>[2x]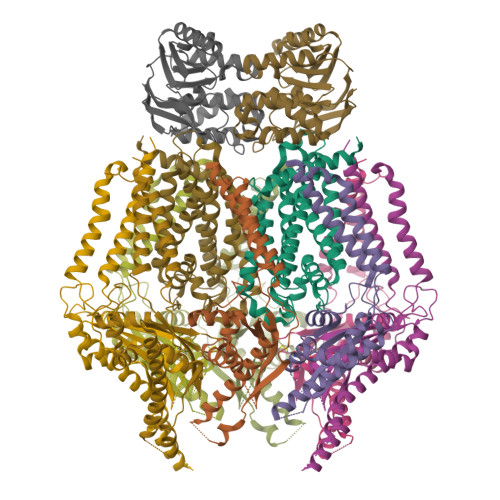MIELRNLTKWYPTPHGRRYVFRNLNFRFPDDVSIGLIGRNGAGKSTLMRLLGGIEAPNEGEVVTDVSISWPVGLSGGFQGSLTARENVKFVCRIYGTSHEDMLRKVRFVEEFAEIGEHFDLPMKTYSSGMRSRVAFGLSMAFDFDYYLIDEAMAVGDAQFRAKSRAVFDSRVGQANMILVSHNMNDIKEYCDVVVLVDQGQATLYEDVEAGIAAYQGSLKKAAAKPDYKDDDDK;>MGKIHLAVSERSPRVKRSPWQIQQAVLFALFLRELKTRLGGRWLGVFWVLLEPVAHIAVMTTLFSLAHRAAMPSIEYPVFLITGLIPFFMFRGLVTRLMEAIDSNRGLFAYRQVKPIDTVIARAMLEISLQSIVYLIALGTLGWLGFHFLPVRALELAGVSAVLIMLGASLGLFFAVVTNEIPQARAIVRISLLPLYFVSGVIFPVHTIPPQYLPLLQLNPVLHLIELSRASFFPQYRVLQGINLAYPAGFALLSLFLALMLYRLRRHQLASVV[2x];>MGKIHMKLVSRLTAKRLQWALVYLPMLVATVYFLVFSADRYVSESVITVRQTSSNAPTGGMSGAALLLAGLTPASREDTCYLQTYIHSMGLLQKLDQQLKLREHFGTPLRDPLFRLWGGTSQEWFLEYYRSRVEVLMDDICGLLTVRVQGFEPEFAQALNRAILEESERFVNELSHRMAREQGQFAEAELERATARLQEAKRQLIAFQAKHKLLDPLAQAQATGTLTAELQAALTRQEAELRNALTYLNEDSYQVKALRSQINALRQQIDEERLRATAGKNGDRINAVAAEFHDLQLQVGFAEDAYKLALAAVESARIEATRKLKSLVVVEPPVLPEIAEYPRRWYNLATLLVVCCLIYGVVSLVVATIRDHQDGSGSGSHHHHHHHHHH[8x]> PKV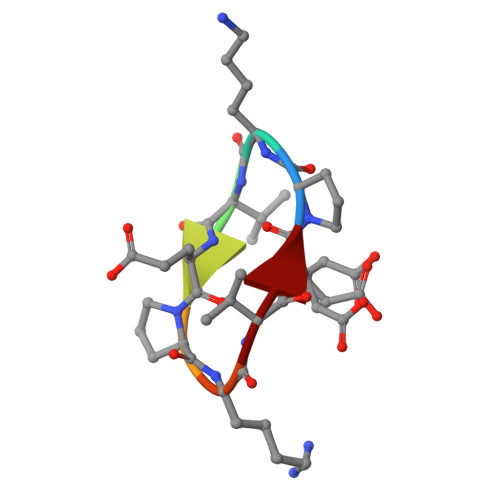EPKVE>[2x]MKFTVEREHLLKPLQQVSGPLGGRPTLPILGNLLLQVADGTL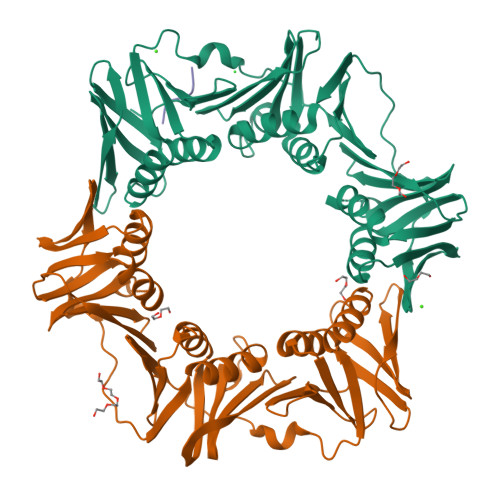SLTGTDLEMEMVARVALVQPHEPGATTVPARKFFDICRGLPEGAEIAVQLEGERMLVRSGRSRFSLSTLPAADFPNLDDWQSEVEFTLPQATMKRLIEATQFSMAHQDVRYYLNGMLFETEGEELRTVATDGHRLAVCSMPIGQSLPSHSVIVPRKGVIELMRMLDGGDNPLRVQIGSNNIRAHVGDFIFTSKLVDGRFPDYRRVLPKNPDKHLEAGCDLLKQAFARAAILSNEKFRGVRLYVSENQLKITANNPEQEEAEEILDVTYSGAEMEIGFNVSYVLDVLNALKCENVRMMLTDSVSSVQIEDAASQSAAYVVMPMRL;> XQLDLA> TGDDKSDEWKKNEWNNWLIKTEEDWKLFNTAVENKKNRWLEKRDKELEVWLMNMQNRWLHYRENEENEYKAEAMKNSATWDDSQWEQWIKTEGKKGMEADLKKWLNDKETFLDGWISKEWVQWKNERMLQWLSVDWKHKEDETFEHYKSSKFTNVLHIKKKKKWTKWKERTNKEKEEWNNWVK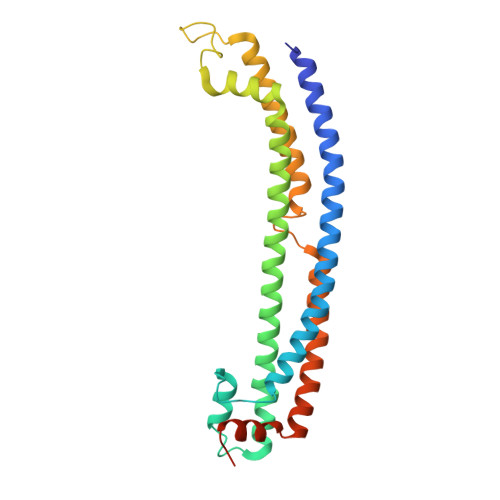GKENLYVNNKWDKWLKWKKDKRALYSQKFLTFINKWISDKQWTVWIEDQGGSTLGTKHHHHHH> MSLAADTPTTCCFSYTSRQIPQNFIADYFETSSQCSKPGVIFLTKRSRQVCAD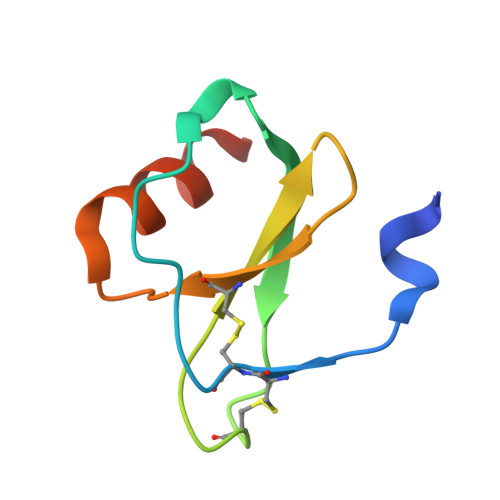PSEEWVQKYVSDLELSA> HHHHHHMKTRIHVVQGDITKLAVDVIVNAANPSLMGGGGVDGAIHRAAGPALLDACLKVRQQQGDCPTGHAVITLAGDLPAKAVVHTVGPVWRGGEQNEDQLLQDAYLNSLRLVAANSYTSVAFPAISTGVYGYPRAAAAEIAVKTVSEFITRHALPEQVYFVC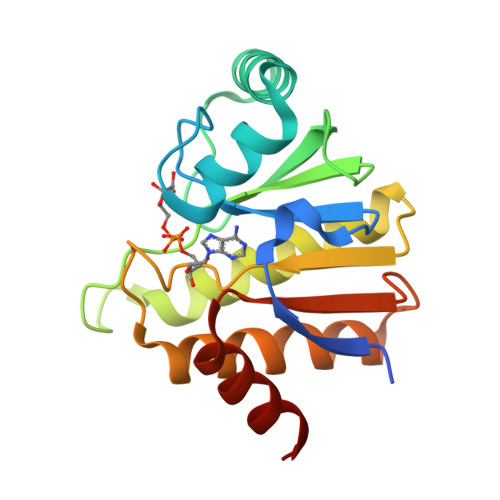YDEENAHLYERLLTQQGDE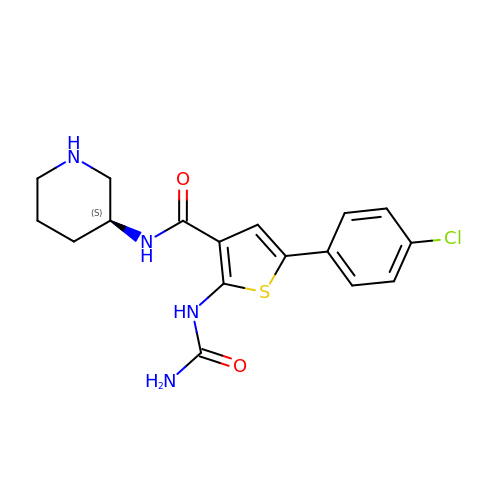2-(carbamoylamino)-5-(4-chlorophenyl)-N-[(3S)-piperidin-3-yl]thiophene-3-carboxamide | C17 H19 Cl N4 O2 S | MZBVMTJFZZINAF-LBPRGKRZSA-N>[4x]MPFVKDFKPQALGDTNLF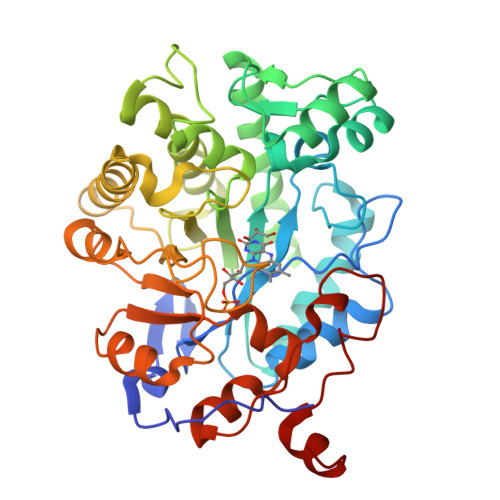KPIKIGNNELLHRAVIPPLTRMRAQHPGNIPNRDWAVEYYAQRAQRPGTLIITEGTFPSPQSGGYDNAPGIWSEEQIKEWTKIFKAIHENKSFAWVQLWVLGWAAFPDTLARDGLRYDSASDNVYMNAEQEEKAKKANNPQHSITKDEIKQYVKEYVQAAKNSIAAGADGVEIHSANGYLLNQFLDPHSNNRTDEYGGSIENRARFTLEVVDAVVDAIGPEKVGLRLSPYGVFNSMSGGAETGIVAQYAYVLGELERRAKAGKRLAFVHLVEPRVTNPFLTEGEGEYNGGSNKFAYSIWKGPIIRAGNFALHPEVVREEVKDPRTLIGYGRFFISNPDLVDRLEKGLPLNKYDRDTFYKMSAEGYIDYPTYEEALKLGWDKN>ETGEVTLLDSRSVQGELGWIASPLEGGWEEVSIMDEKNTPIRTYQVCNVMEPSQNNWLRTDWITREGAQRVYIEIKFTLRDCNSLPGVMGTCKETFNLYYYESDNDKERFIRENQFVKIDTIAADESFTQVDIGDRIMKLNTEIRDVGPLSKKGFYLAFQDVGACIALVSVRVFYKRTKHHHH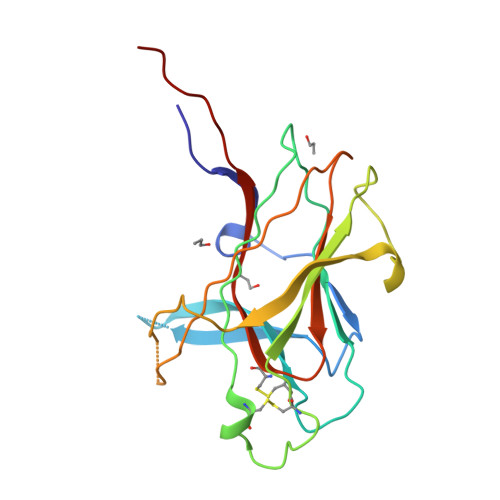HH[2x]> NLIRKNVDTLTPDEILNLQVSLRAMQDDEGASGYQAISAYHGEPADCKAADGSTIVCCLHGMPTFPMWHRLYLVQFEQALVAHGSTLGIPYWDWTKPMTQLPELVQHPLFIDPTGKKAKKNVFYSGEIKFENKVTARAVDARLYQASQEGQKNFLLEGVLNALEQEDFCHFEVQLEVAHNPIHYLVGGRFTHSMSSLEYTSYDPLFFLHHSNVERHFALWQALQKHRGLPTRPNCGLNLFHSPMEPFGRDTNPFAITKDNSKASSLFDYEHLGYAFDDLSLNGMTIEELEALLKQ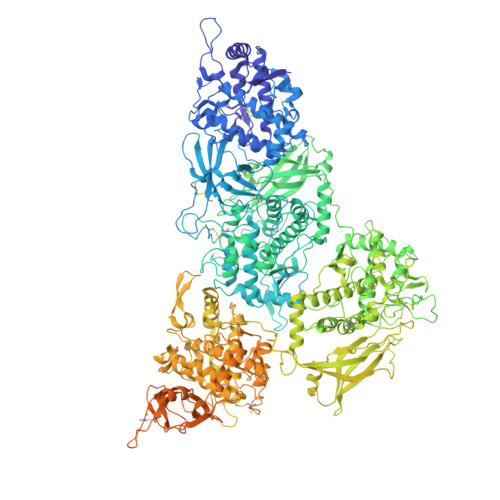RRSGARAFANFRLGGIKTSANVRIKLCIPTEDKRQSDNCDNDAGQFFILGGTNEMPWNFAFPYLHEITDTVLSLGLALDSNYYVTAEVTAINGTLMPTQTIPRPIVTYIPPQGFKDVNMVNMDTSSLRFRKDISSLTTEEEYELRVAMERFMSDKSINGYQALAEFHGLPAKCPRPDALNRVACCIHGMATFPHWHRLVVMQFENALFTRGSPIGVPYWDWTKPFTALPSLLADETYVDPYTKETKPNPFFKAPIEFLKAGVHTSRQIDERLFKQPSKGDHGFLYDGLSLAFEQDDFCDFEVQFEVTHNSIHAWTGGSEPYSMSSLHYTSFDPMFWLHHSQVDRLWAIWQALQIQRGKPYKTYCANSEVYRPMKPFAFKSPLNNDEKTREHSVPTDVYDYQAELAYTYDTLFFGGLSIRELQRYVEEAKSKDRVFAGFLLMGIQTSANVDLFVVAGGNEFFVGSIAVLGGSKEMTWRFDRVYKHEITDALGALGVDMFAEYTLRVDIKDVNGTALPPTAIPPPIVIFVPGIADANVKFDEQHRSRKNVDSMTVSEMNALRTAMAAFAADKEVTGYQQVAAFHGSTQWCPSPDAAQKYACCHHGMATFPHWHRLIALNFENGLRRNGWSGGLPYWDWTRPIDALPALVLEAEYTDANGEAKPNPFFSGAIDSIGASTSRAPTEALYEKPDFGKYTHLANEIISALEQEDFCDFEVQYEIAHNHIHALVGGTEAVSMASLEYSAFDPIFMLHHSNVDRIWATWQALQKFRGKAYNSANCAIEILRKPMSPFSLASDINPDAMTREYSVPFDVFNYKKNFHYEYDTLELNGLSIAQLSREINRRKAKNRVAVTFMLEGLKKSLLVEYFIAADGTDQKMKAGEFYVLGSENEMPWKFDRPYKSDITYVMDAMKLHYTDKYHVELRITDMTGAEVTDLKLVTSVIYEPGIGNFGEGRRWISPITSASRIRKNLLDFEDGEMESLRNAFKQMADEGRYEEIASFHGVPAQCPSEDGTMVHTCCLHGMPVFPHWHRLYVSLVEDELLARGSGVAVPYWDWVEPFDELPRLINEATFYNSRTLQIEPNPFFKGKISFENAETDRDTQPELFGNRYLYDHTLFVFEQTDFCEFEVHYEVLHNTIHSWLGGRDVHSMSSLDYAAYDPVFFLHHSNVDRLWAIWQELQRYRKLSYNEANCALPLMNQPMRPFSNSTANNDRLTFTNSRPNDVFDYQNVLHYKYDTLNFAGLSIPQLERILQKNQGRDRIFAGFLLHGIKASADVRIYICVPTGIGEENCGNYAGIFSVLGGETEMPWQFDRLFRYEITDELKKLGLNQNSHFRVEMELTAVNGSKITQKIFPNPTIIFVPSDVEFEEDTWRDVVTSANRIRRNLKDLSKEDMFSLRAAFKRMTDDGRYEEIAAFHGLPAQCPNADGSNIHTCCLHGMPTFPHWHRLYLSLVENELLARGSDVAVPYWDWIEPFDSLPGLISDETYKHPKTNEDIENPFHHGKISFADAVTVRKPRDQLFNNRYLYEHALFAFEHTDFCDFEVHFEVLHNSIHSWIGGPNPHSMSSLDFAAYDPIFFLHHSTVDRLWAIWQDLQRYRKLDYNVANCALNLLNDPMRPFNNKTANQDHLTFTNSRPNDVFDYQNSLNYKFDSLSFSGLSIPRLDDLLESRQSHDRVFAGFWLSGIKASADVNIHICVPIGVEHEDCDN> EGFKANLSLLRRPGEKTYTQRCRLFVGNLPADITEDEFKRLFAKYGEPGEVFINKGKGFGFIKLESRALAEIAKAELDDTPMRGRQLRVRFATHAAALSVRNLSPYVSNELLEEAFSQFGPIERAVV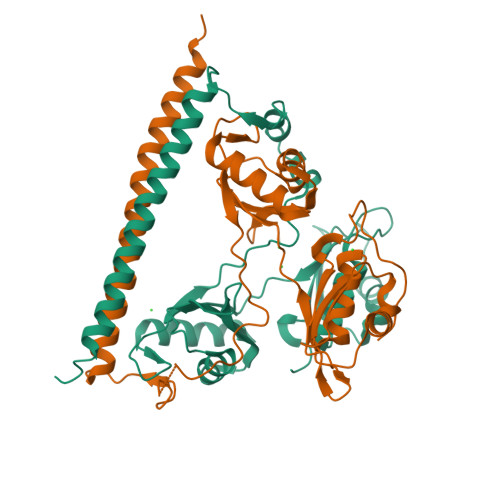IVDDRGRSTGKGIVEFASKPAARKAFERCSEGVFLLTTTPRPVIVEPLEQLDDEDGLPEKLAQKNPMYQKERETPPRFAQHGTFEYEYSQRWKSLDEMEKQQREQVEKNMKDAKDKLESEMEDAYHEHQANLL;> EGLTIDLKNFRKPGEKTFTQRSRLFVGNLPPDITEEEMRKLFEKYGKAGEVFIHKDKGFGFIRLETRTLAEIAKVELDNMPLRGKQLRVRFACHSASLTVRNLPQYVSNELLEEAFSVFGQVERAVVIVDDRGRPSGKGIVEFSGKPAARKALDRCSEGSFLLTTFPRPVTVEPMDQLDDEEGLPEKLVIKNQQFHKEREQPPRFAQPGSFEYEYAMRWKALIEMEKQQQDQVDRNIKEAREKLEMEMEAARHEHQVMLM>[24x]EEAELAYLLGELAYKLGEYRIAIRAYRIALKRDPNNAEAWYNLGNAYTKQGDYDEAIEYYLRALVLDPNNAEAATNLGQAYMNQGDKDRAKLMLLLALKLDPNNDSARVILGVAKVGIEELAKLASQAQQEGDSEKQKAIELAAEAARVAQEVGDPELEKLALEAARRGDSEKAKAILLAAEAARVAKEVGDPELIKLALEAARRGDSEKARAILEAAERAREAKERGDPEQIKKARELAKR;>[24x]DVSALAYVMLGLLLSLLNRLSLAAEAYKKAIELDPNDALAWLLLGSVLEKLKRLDEAAEAYKKAIELKPNDASAWKELGKVLEKLGRLDEAAEAYLIAIMLDPEDAEAAKELGKVLEKLGELEMAEEAYKLAIKLDPND

Computationally designed multi-subunit assemblies have shown considerable promise for a variety of applications, including a new generation of potent vaccines. One of the major routes to such materials is rigid body sequence-independent docking of cyclic oligomers into architectures with point group or lattice symmetries. Here we describe RPXDock, a fast, flexible, and modular software package for sequence-independent rigid-body protein docking across a wide range of symmetric architectures that is easily customizable for further development. RPXDock uses an efficient hierarchical search and a residue-pair transform (RPX) scoring method to rapidly search through multidimensional docking space.

We set out to experimentally evaluate symmetric one- and two-component structures with polyhedral group symmetry generated using RPXDock. Given a set of prevalidated homomeric scaffolds with cyclic symmetry, we generated docks using RPXDock, and the resulting interfaces were sequence-optimized via Rosetta sequence design. E. Characterization of the two-component octahedral assembly O43-rpxdock-EK1 by cryogenic electron microscopy. To the right are representative 2D class averages showing different axes of symmetry and a reconstructed 3D map at 3.7 Å resolution. The overlay of the original dock (orange and purple) with the model built from the 3D reconstruction (gray) shows 4 Å Cα root mean square deviation between the original dock and cryoEM structure over 48 chains. Local resolution estimates range from ~3.2 Å at the core to >4.0 Å along the periphery of the extended arms due to a high degree of flexibility within this region. The protruding arms of the designed cage only start to become visible at very low contour levels.> MIALGLGLGLAANGGPALRRYAVNGVAPVAVLDFERHFLSHPLALTRATSATYADALRAVQTAPADTPRYDYSTGKRALLLEASATNLLPNSAQFEAASWGKTRASVLANAALAPNGTMTADKLVEDTSNNSHFVARTGTQIAAGTSVTASIFVKAAERRWFALVTADSANAFRTTYFDLQTGTLGVVSQGAAGHVAQIVAAGNGWYRCSVTQTQAASGNFNFYPSVASANGATSYPGDGASGLYLWGAQLEAGAAVSSVIPTEAAAVTRAADLASVAVAAGSYDLRRVDAAGTAVTKGVA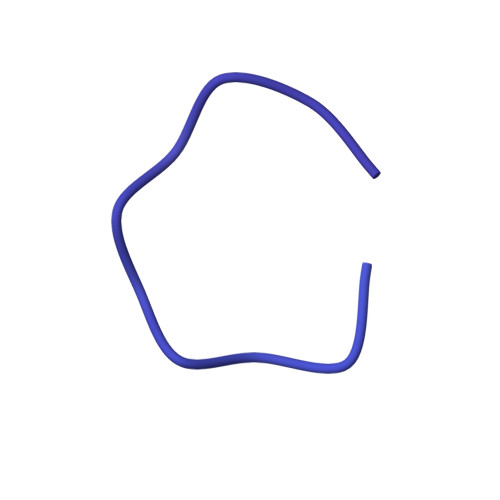HPGGALTIGAGSLYLLSLFPAGAL>[2x]MHVIKRDGRQERVMFDKITSRIQKLCYGLNMDFVDPAQITMKVIQGLYSGVTTVELDTLAAETAATLTTKHPDYAILAARIAVSNLHKETKKVFSDVMEDLYNYINPHNGKHSPMVAKSTLDIVLANKDRLNSAIIYDRDFSYNYFGFKTLERSYLLKINGKVAERPQHMLMRVSVGIHKEDIDAAIETYNLLSERWFTHASPTLFNAGTNRPQLSSCFLLSMKDDSIEGIYDTLKQCALISKSAGGIGVAVSCIRATGSYIAGTNGNSNGLVPMLRVYNNTARYVDQGGNKRPGAFAIYLEPWHLDIFEFLDLKKNTGKEEQRARDLFFALWIPDLFMKRVETNQDWSLMCP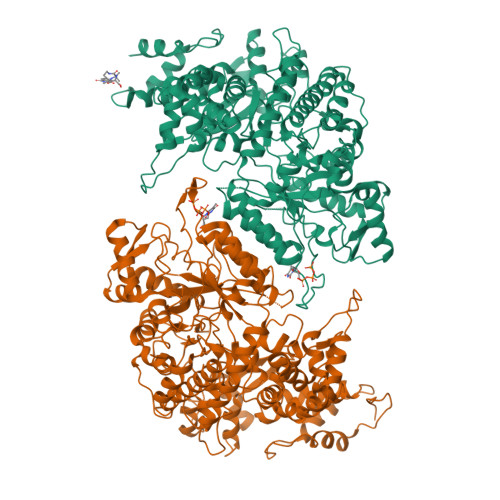NECPGLDEVWGEEFEKLYASYEKQGRVRKVVKAQQLWYAIIESQTETGTPYMLYKDSCNRKSNQQNLGTIKCSNLCTEIVEYTSKDEVAVCNLASLALNMYVTSEHTYDFKKLAEVTKVVVRNLNKIIDINYYPVPEACLSNKRHRPIGIGVQGLADAFILMRYPFESAEAQLLNKQIFETIYYGALEASCDLAKEQGPYETYEGSPVSKGILQYDMWNVTPTDLWDWKVLKEKIAKYGIRNSLLIAPMPTASTAQILGNNESIEPYTSNIYTRRVLSGEFQIVNPHLLKDLTERGLWHEEMKNQIIACNGSIQSIPEIPDDLKQLYKTVWEISQKTVLKMAAERGAFIDQSQSLNIHIAEPNYGKLTSMHFYGWKQGLKTGMYYLRTRPAANPIQFTLNKEKLKDKEKVSKEEEEKERNTAAMVCSLENRDECLMCGS>[4x]GSHMASPSNTDYPG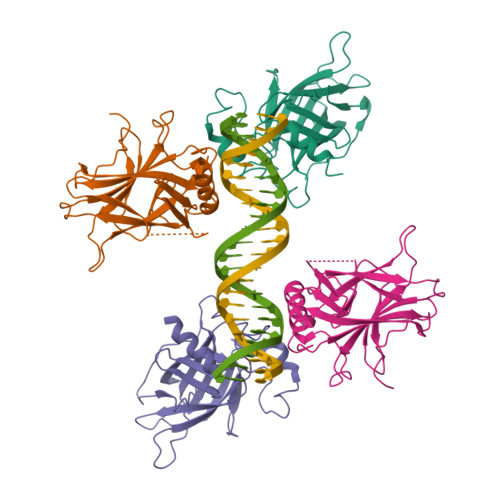PHSFDVSFQQSSTAKSATWTYSTELKKLYCQIAKTCPIQIKVMTPPPQGAVIRAMPVYKKAEHVTEVVKRCPNHELSREFNEGQIAPPSHLIRVEGNSHAQYVEDPITGRQSVLVPYEPPQVGTEFTTVLYNFMCNSSCVGGMNRRPILIIVTLETRDGQVLGRRCFEARICACPGRDRKADEDSIRKQ The Arabidopsis immune receptors RRS1 and RPS4 detect the Pseudomonas syringae pv. pisi secreted effector AvrRps4 via a WRKY ID in RRS1. RRS1-R contains an integrated WRKY domain near its C terminus (RRS1WRKY), which interacts with two structurally distinct type III secreted bacterial effectors, AvrRps4 from P. syringae pv. pisi and PopP2 from R. solanacearum. The RRS1WRKY domain may mimic the DNA-binding domain of WRKY transcription factors (TFs), the putative virulence targets of AvrRps4 and PopP2, to enable immune perception of these effectors. AvrRps4 is proteolytically processed in planta to produce a 133–amino acid N-terminal fragment (AvrRps4N) and an 88–amino acid C-terminal fragment (AvrRps4C).

To reveal the molecular basis of the AvrRps4C and RRS1WRKY interaction, we coexpressed the proteins in E. coli, purified the complex, and obtained crystals that diffracted with 2.65-Å resolution at the Diamond Light Source. The structure comprises a 1:1 complex of AvrRps4C and RRS1WRKY, which supports the 1:1 binding model in ITC. The binding interface between AvrRps4C and RRS1WRKY is largely formed by residues from the β2-β3 strand of RRS1WRKY, which present a positive surface patch that interacts with acidic residues on the surface of AvrRps4C. The characteristic WRKY sequence signature motif WRKYGQK maps to the β2-strand of RRS1WRKY and is directly involved in contacting AvrRps4C. The interaction between the β2-segment of RRS1WRKY, which harbors the WRKYGQK motif, and AvrRps4C includes hydrogen bonds and/or salt-bridge interactions involving Tyr1218 and Lys1221 of RRS1WRKY and AvrRps4 Glu175, Glu187, and Asn171. Notably, the side chain of RRS1WRKY Lys1221 protrudes into an acidic cleft on the surface of AvrRps4C to contact the side chains of both AvrRps4 Glu175 and Glu187. The complex between AvrRps4C and RRS1WRKY is further stabilized by the β3-strand of RRS1WRKY that forms hydrogen bonds and salt-bridge interactions via side chains of RRS1WRKY Arg1230, Tyr1232, and Arg1234 to AvrRps4 Glu175 and Asp164. We found that mutating AvrRps4 residues Asp164 (D164A), Glu175 (E175A), Glu187 (E187A), and double mutant Glu175/Glu187 (EE/AA) essentially abolished complex formation in vitro. The structure of the AvrRps4C–RRS1WRKY complex reveals that the effector directly interacts with the DNA-binding WRKYGQK motif, likely rendering it unavailable for binding to DNA. Comparing the AvrRps4C–RRS1WRKY structure with that of PopP2–RRS1WRKY reveals an overlapping binding site for the effectors, primarily mediated by the β2-β3 segment of the WRKY domain.

> GPGKRVYQIGSSSRDVQVCPRGAGAALRQEIEDKQLMVNNLTDELQDAIDEANPAEIANTSQQLRHARADLADLQRRFAVLRNEDRRINQ;> SESKVKKVVSIPAIDEGDLWTWRKYGQKDILGSRFPRGYYRCAYKFTHGCKATKQVQRSETDSNMLAITYLSEHNHPRPT(5R)-5-[(5-methoxy-3-oxo-1,3-dihydro-2H-indazol-2-yl)methyl]-5-methylimidazolidine-2,4-dione | C13 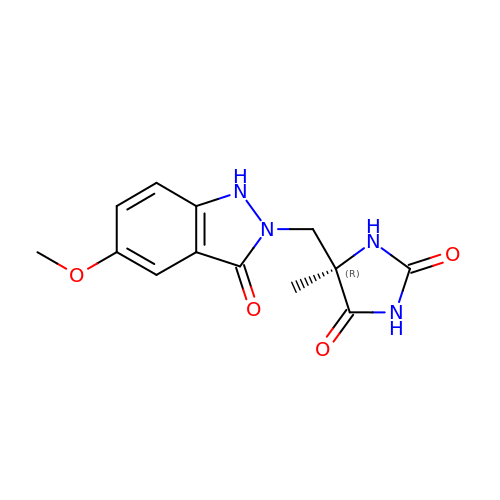H14 N4 O4 | PIEMRKVLYXWKFP-CYBMUJFWSA-N>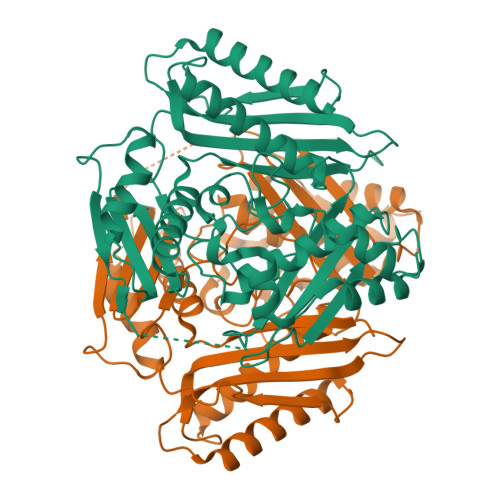[4x]MQYKKIITSESVGAGHPDKICDQISDAILDECLSQDQNSRVACEVLACNRLIVIAGEITTHAYVDVVKTAWEIIKPLGYDENDFTIISNVNKQSVDIAQSVDKTNKNLIGAGDQGIVFGYACDETPQYMPLTSVLAHELLKEIERQRRSKEFIKIQADMKSQVSIDYSNSTPLIETMLVSIQHDEDYDVEYFNKKVSAIMEQIAKKYNLNTNFKKIINSSGRFVIGGPIGDTGLTGRKIIVDTYGGVGHHGGGAFSGKDPTKVDRSASYFARWIAKNVVAAKLAKQCEIQLAFAIGQPQPVAMYVNTFNTNLIDETKIFEAIKKSFNFDIKTFINDLNLWTTKYLPVATYGHFGRDDLDLSWEKLNKVEDLIKNSKHHHHHH> GAAAQGTVRKAGALAVKNFLVHKKNKKVESATRR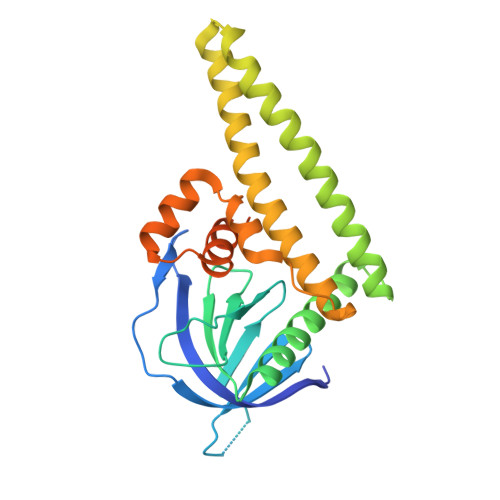KWKHYWVSLKGCTLFFYESDGRSGIDHNSIPKHAVWVENSIVQAVPEHPKKDFVFCLSNSLGDAFLFQTTSQTELENWITAIHSACATAVARHHHKEDTLRLLKSEIKKLEQKIDMDEKMKKMGEMQLSSVTDSKAAATILDQIFVWEQNLEQFQMDLFRFRCYLASLQGGELPNPKRLLAFASRPTKVAMGRLGIFSVSSFHALVAARTGETGVRRRTQAMSRSASKRRSRFSSLWGLDTT>DSVSQCFFDYYTSKILIIRSKKVGTLNRFTQALVIAYVIGYVCVYNKGYQDTDTVLSSVTTKVKGIALTNTSELGERIWDVADYIIPPQEDGSFFVLTNMIITTNQTQSKCAENPTPASTCTSHRDCKRGFNDARGDGVRTGRCVSYSASVKTCEVLSWCPLEKIVDPPNPPLLADAENFTVLIKNNIRYPKFNFNKRNILPNINSSYLTHCVFSRKTDPDCPIFRLGDIVGEAEEDFQIMAVRGGVMGVQIRWDCDLDMPQSWCVPRYTFRRLDNKDPDNNVAPGYNFRFAKYYKNSDGTETRTLIKGYGIRFDVMVFGQAGKFNIIPTLLNIGAGLALLGLVNVICDWI[3x]

P2X receptors are ATP-activated cation channels, and the P2X4 subtype plays important roles in the immune system and the central nervous system, particularly in neuropathic pain. Here, we report the cryo-EM structures of the zebrafish P2X4 receptor in complex with two P2X4 subtype-specific antagonists, BX430 and BAY-1797. Both antagonists bind to the same allosteric site located at the subunit interface at the top of the extracellular domain. The overall structures of the zebrafish P2X4 receptor in complex with BX430 and BAY-1797 are very similar and show a chalice-like trimeric architecture with each subunit containing a relatively large extracellular domain and two TM helices, resembling the shape of a dolphin, as in the previously reported P2X receptor structures.

BX430, or 1-(2,6-dibromo-4-isopropylphenyl)-3-(3-pyridyl)urea, is a phenylurea antagonist. BX430 inhibited ATP-dependent currents of both zebrafish P2X4 and human P2X4 (hP2X4) with comparable IC50 values at sub-micromolar levels, and the results were consistent with the previously reported IC50 value of 0.54 µM for hP2X4. In the BX430-bound structure, the dibromo-isopropylphenyl group of BX430 faces the outer side of the receptor, while the pyridine group faces the inner side. The binding site consists mainly of hydrophobic residues, including Trp87, Ile94, Met108, Ile110, Phe299, and Ile315 from one subunit and Tyr302 from the neighboring subunit. In addition, the main chain carbonyl group of Asp91 forms hydrogen bonds with the amines in the urea group of BX430. Interestingly, the side chain of Lys301 forms a cation-pi interaction with the aromatic ring of Tyr302 from the neighboring subunit, allowing hydrophobic interactions between the side chain of Lys301 and the 4-isopropylphenyl ring of BX430. Furthermore, there are intersubunit salt bridges between the side chains of Arg85 of one subunit and Glu310 of the neighboring subunit, and hydrogen bonds between the side chain of Tyr302 of one subunit and the main-chain carbonyl group of Ala90 and the side chain of Asp91 of the neighboring subunit. Further close inspection of the allosteric site revealed that in the apo state, the side chain of Lys301 faces the inside of the receptor, which would cause steric hindrance with the pyridine group of BX430 in the BX430-bound structure. It should be noted that the binding pocket is more expanded in the presence of BX430 than in the presence of BAY-1797, probably simply because the 4-isopropylphenyl ring of BX430, located in the outer region of the binding pocket, is bulkier than the phenyl ring of the phenylacetamide moiety of BAY-1797.>SMRKKIFKPEELRQALMPTLEALYRQDPESWPFRQPVDPQLLGIPDYFDIVKNPMDLSTIKRKLDTG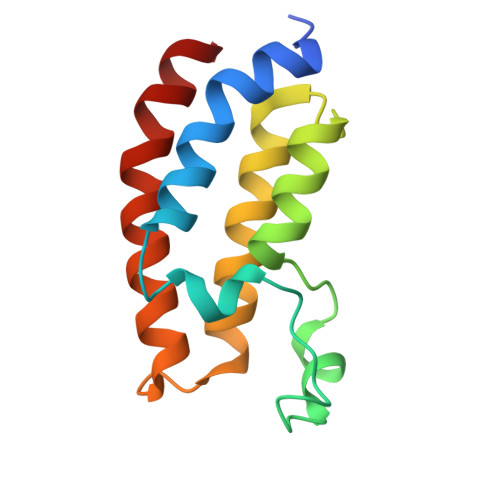QYQEPWQYVDDVWLMFNNAWLYNRKTSRVYKFCSKLAEVFEQEIDPVMQSLG[2x]> HTVELNEMFGQIQSPGYPDSYPSDSEVTWNITVPEFRVQLYFMHFNLESSYLCEYDYVKVETEDQVLATFCGRETTDTEQTPGQEVVLSPGSFMSVTFRSDFSNEERFTGFDAHYMAVDVDECKEREDEELSCDHYCHNYIGGYYCSCRFGYILHTDNRTCRVECSGNLFTQRTGTITSPDYPNPYPKSSECSYTIDLEEGFMVTLHFEDIFDIEDHPEVPCPYDYIKIKAGSKVWGPFCGEKSPEPISTQSHSIQILFRSDNSGENRGWRLSYRA

The lectin pathway of complement is activated by complexes comprising a recognition component (mannose-binding lectin, serum ficolins, collectin-LK or collectin-K1) and a serine protease (MASP-1 or MASP-2). MASP-1 activates MASP-2, and MASP-2 cleaves C4 and C4b-bound C2. MASPs are homodimers that circulate as zymogens bound to the collagenous domains of MBL. Each MASP comprises two N-terminal CUB (C1r/C1s, Uegf, and bone morphogenetic protein-1) domains separated by an epidermal growth factor (EGF)-like domain followed by two short complement regulator (SCR) domains and a C-terminal serine protease (SP) domain.

Because there was no structure of rat MASP-1 3D, and the existing structure of rat MASP-2 3D lacked two of the three Ca2+, including those Ca2+ that form part of the binding site for MBL, both rat MASP-1 3D and MASP-2 3D were crystallized in the presence of 2 mM calcium and diffraction data were collected. This resulted in one MASP-1 structure at 3.7 Å resolution and three independent MASP-2 structures at 2.6–2.7 Å resolution. For MASP-1 3D, 276 of its 281 residues could be built into the electron density map. All four crystal structures revealed a dimer of MASP-1 3D or MASP-2 3D, formed by antiparallel neighboring contacts between pairs of CUB1-EGF domains about the crystallographic symmetry axis. The total buried surface area for MASP-1 at the dimer interface was 880 Å2 per molecule (1,760 Å2 in total), whereas the three crystal structures for MASP-2 gave 1,200, 1,090, and 950 Å2 per molecule. All four new crystal structures revealed well-ordered, similar calcium-binding sites in each of the CUB1 and CUB2 domains. In the MASP-1 CUB1 domain, Ca2+ formed contacts with six oxygen atoms in the side chains of Glu49, Asp57, Asp102, Ser104, and Asn105 (distances between 2.3 and 2.4 Å). In the MASP-1 CUB2 domain, Ca2+ now formed contacts with five oxygen atoms in the structurally equivalent side chains of Glu216, Asp226, Asp263, and Ser265. The EGF domains of MASP-1 and MASP-2 also bound calcium. Interestingly, the prediction of 4.26 S from the MASP-1 3D crystal structure was similar to the observed value of 4.53 ± 0.08, while that of 4.18 S from the MASP-2 crystal structure was close to the observed value of 4.09 ± 0.07 S.> XYRIPSYDFADEAEKLLRDAAG;> XYR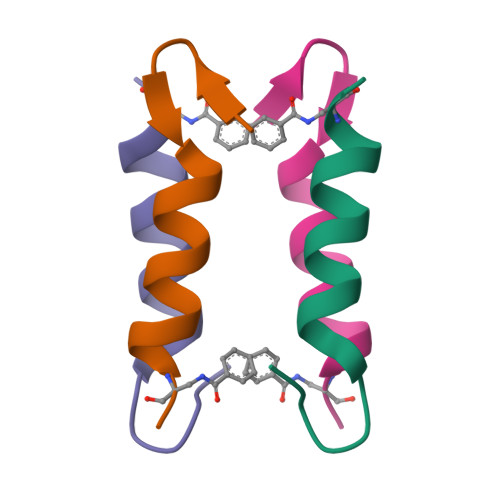IPSYDFADKFKKLLRKAAG> MLVELLEFTPLSFIDDVINITNQLLYKGVNGVDKAFSQTRFAKKAPQEIEEGLHKFEVLFESVVDRYYDGFEVYTLRNIFSYPPELKGYMRTFGKDVDYSIT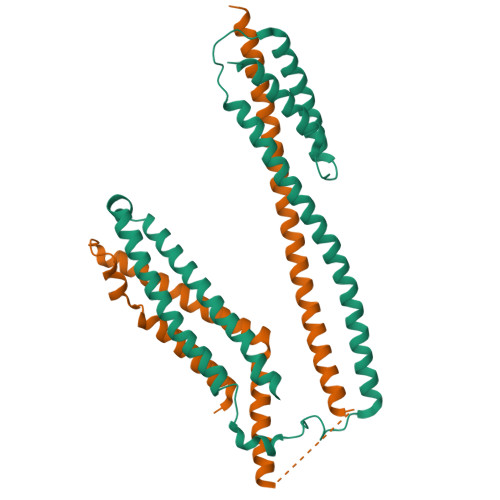TEQDAAMDQAIQEAAEKLVVKMQLRRDLRMRLSRKREKKTEIEKHLERISFLNKVPENWQVTLPETTDFLLDQLGNLQHAVKRVVEASPTVHSREVDERITYLEKGYERLSNP;> MTSRKEQLDAFLSRTLSETIAHIPLEKFAQCFPSMKKGKVIAVIHQQLIEFFEKSCKQEYANLIKERDLNKKLDMLDECIHDAEFRKLHGESEVDISNKQPQEILKAHLYSHKRELLDKLNQDLLDIDKENEGLSTQIAAEEKATEDCISRMQSLIQKLEKTVYGMNEKNLAKEA> MSQQVDKIKASYPLFLDQDYKDMLAKKRDGFEEKYPQDKIDEVFQWTTTKEYQELNFQREALTVNPAKACQPLGAVLCALGFEKTMPYVHGSQGCVAYYRSYFNRHFREPVSCVSDSMTEDAAVFGGQQNMKDGLQNCKATYKPDMIAVSTTCMAEVIGDDLNAFINNSKKEGFIPDEFPVPFAHTPAFVGSHVTGWDNM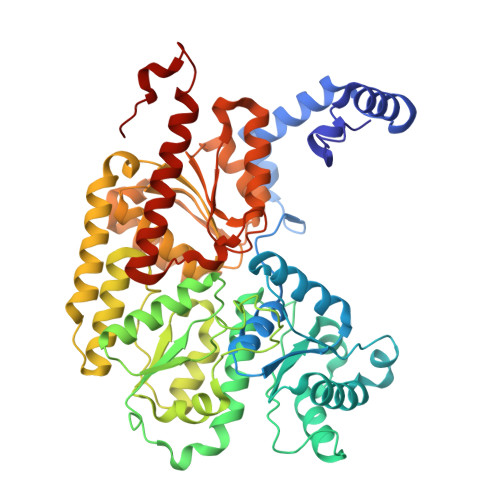FEGIARYFTLKSMDDKVVGSNKKINIVPGFETYLGNFRVIKRMLSEMGVGYSLLSDPEEVLDTPADGQFRMYAGGTTQEEMKDAPNALNTVLLQPWHLEKTKKFVEGTWKHEVPKLNIPMGLDWTDEFLMKVSEISGQPIPASLTKERGRLVDMMTDSHTWLHGKRFALWGDPDFVMGLVKFLLELGCEPVHILCHNGNKRWKKAVDAILAASPYGKNATVYIGKDLWHLRSLVFTDKPDFMIGNSYGKFIQRDTLHKGKEFEVPLIRIGFPIFDRHHLHRSTTLGYEGAMQILTTLVNSILERLDEETRGMQATDYNHDLVR> GPLGSMSQSNRELVVDFLSYKLSQKGYSWSQMAAVKQALREAGDEFELRYRRAFSDLTSQLHITPGTAYQSFEQVVNELFRDGVNWGRIVAFFSFGGALCVESVD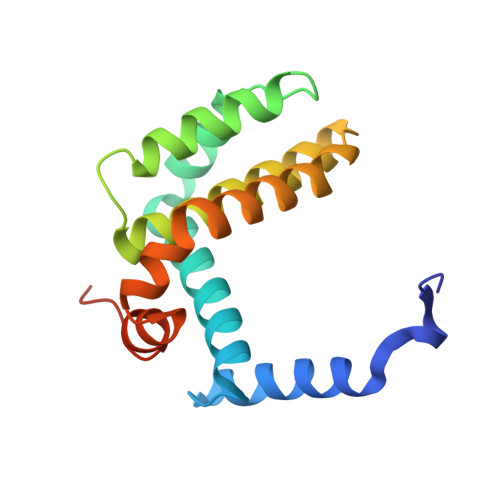KEMQVLVSRIAAWMATYLNDHLEPWIQENGGWDTFVELYGNNAAAESRKGQER>GSVIDPSELTFVQEIGSGQFGLVHLGYWLNKDKVAIKTIREGAMSEEDFIEEAEVMMKLSHPKLVQLYGVCLEQAPICLVFEFMEHGCL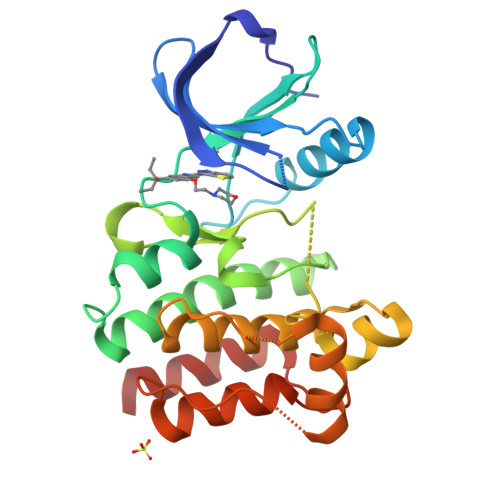SDYLRTQRGLFAAETLLGMCLDVCEGMAYLEEACVIHRDLAARNCLVGENQVIKVSDFGMTRFVLDDQYTSSTGTKFPVKWASPEVFSFSRYSSKSDVWSFGVLMWEVFSEGKIPYENRSNSEVVEDISTGFRLYKPRLASTHVYQIMNHCWKERPEDRPAFSRLLRQLAEIAESGL[2x]(3R)-3-[(1,2,3,4-tetrahydroisoquinolin-7-yloxy)methyl]-2,3-dihydrothieno[2,3-f][1,4]oxazepin-5-amine 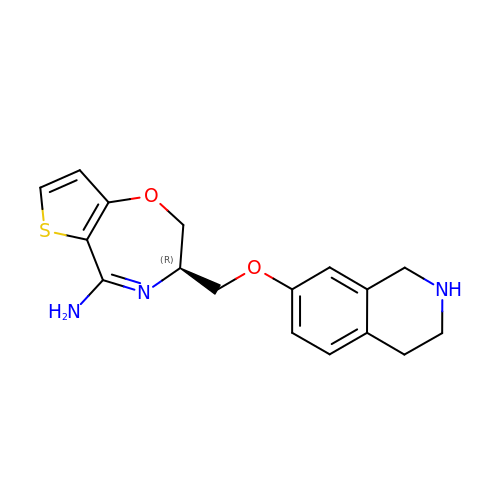| C17 H19 N3 O2 S | UDFXWCLBONUMNA-CYBMUJFWSA-N>MSAKNNTHHFPKLLILVGAPGSGKSTFARYFIRTEDNWVRVNRDDFRLMQFGDSLMSPFYEERITKMVEASVIALLKNRTNVIIDATNSSLRSLQDMVHTYTEYADISFKVFDLPVEELVKRCDKRCEQTGKFIPKSAIEKHVTQLQYTKEKFDFKPIPRALKETSLTYADQDTSLPKAVICDLDGTLSLLNGRDPYNASTADQDLLNTPVAMVLKMAKQQGYKVILLSGRENAYREPTERFLAKYQIDYDLLLMRDTNDYRKDNIIKKELFLEEIQGKYFVEFLLDDRNQVVDMWRRELALPCFQVNYGDF[2x];>[2x]MEDKTLIKKRIDWFCKNKINAFSPTISPAPKSVERNEIESLYEGILWFVLNGVKEIVIEKKYMGSYCDIYLHRRLEDTYLVSRNGYKINHLDQEQCLRALQGLHDRFSWDGVELRIIQSELMPWSILGKGLINNEFSAYYISHEIHAEYLVQSSLYEKLQKIQQEPAYLSFVADAKVLSAKELKDKYPMHIIRQYQSIRDFKFLDLPHYQQNIQLFKRQLDIFGKEAAPFFKPFNILKEVYTDGREHFVNDNLSFQQINDDDFLHYQFTDREDFEAKYPQIRAWVDQVNQSDEEGVVIKPRTAFLPGMPPAFKVRNNDYLTLVYGVDFEDRLQEQIAKRNIKGKLRCSINDWAINAKLLAIPYSELGEENYELKNLVLDRILGEEIENQLDSRL;>MILQIHSQNPHLLDLLNKNPHTDLGIYAKSLRNGQLIGNAVSAYQYDVVFQDTRYSYLPEESNQIDFQSYCSPLVILHICNEFFKELLQEKQTYWSQQIKWLERTRAEVDTYPCTIEVKNLYANSTWYSKGHFMMERYFKNIHITPIVGNNLSLRVEGKSVFEAMNLLSFIAVTTHITNTYGEYTYIDDHFAQKYARILTNIPQVPYFVFYLFIKRAIKSERQFAEIKPMFEAYFKEEGLDIDFQFTDTHGSRMDFIVKELGMEYPILDIGCGELKYYRRFMRRNYNYSHPYFATDTDKSVGDYAALLKERMEADNLYFFSDWTDYEYKNPVNIILTEVIEHNTPEAAEALVKHCLSLNFHKMIITTPNSLFNKYYFDEDPESLRHEDHHFEWTPQEFQDFIRHCVGDTSLEVT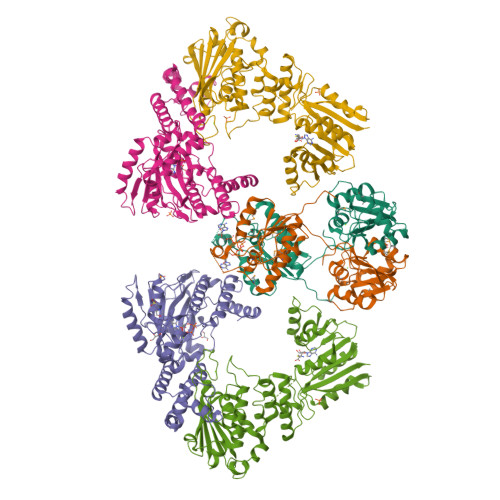YCGIGDRINGETPTQAVVITRK[2x]> MSTPAPPEEQARLLEDALIAVRQQTAMMRKFLDTPGKLMDALKCCSTLVSELRTSSLSPKQYYELYMAVFDALRYLSAHLRENHPVNHLADLYELVQYAGNIIPRLYLMITVGTAYMSIDGAPVKELMKDMMDMSRGVQHPVRG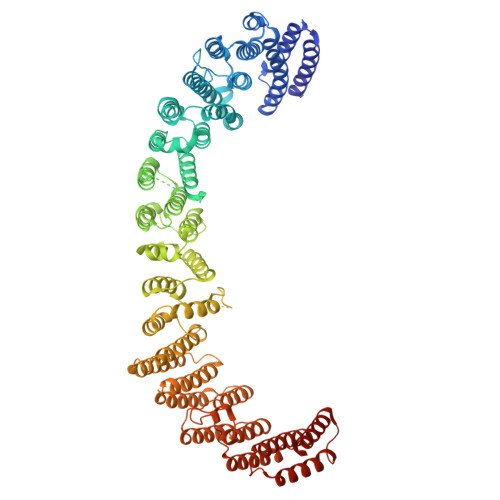LFLRYYLSGQARDYLPTGDSDGPEGNLQDSINFILTNFVEMNKLWVRLQHQGHSRERDLRTQERRELQLLVGSNIVRLSQLVDLPTYRDSILGPLLEQIVQCRDILAQEYLLEVITQVFPDEYHLHTLDQFLGAVSRLNPHVNVKAIVIGMMNRLSDYAERESQNEPEEDRAKLEEEALAKLLEKTKLGQNSELEPQNGDHPDTEVSSTTDSAQAPSTADSDTTAVNGEEEPVRKRRGIPVNVPLYDIFFDQVQHLVQAQHLPIQDTIALCCSLANLSLNIYPERLDYVDGILAYALAKVKEHANSADLHSQPAQQSLLSLLQSPLRRYVSIFTALSLPTYVSLFQAQTYPTRRAIAGEIVRTLLKNQTLISTPAHLENVLEILKVLIKEGSQPPAGYPGVVQPRARPLETDETMEEQGWLARLVHLIHSDDNDTQFRLLQMTRKAYAEGNERIRTTTPPLITAGLKLARRFKAREHYDDNWSSQSSSLFKFLHSAISTLYTRVNGPGVADLCLRLFCSCGQVADMTEFEEVAYEFFAQAFTVYEESISDSKAQFQAVCVIASALHRTRNFGRENYDTLITKCAQHASKLLRKPDQCRAVYLASHLWWATPIAARGETEDTELYRDGKRVLECLQRALRVADSCMETATSIELFVEILDRYVYYFDQRNESVTTKYLNGLIELIHSNLAGNQQDSASVEASRKHFIQTLEMIQSKEFEGIVVAPK>[2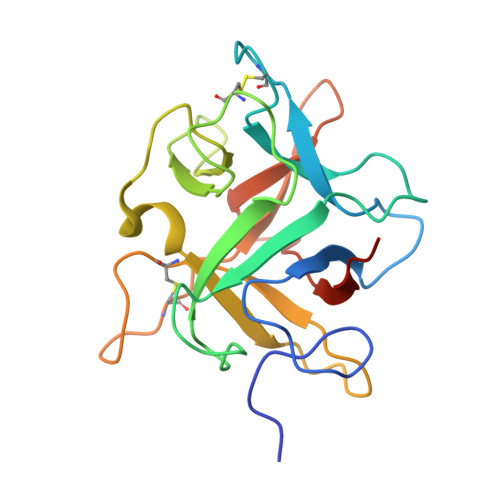x]GSHMDDDLVDAEGNLVENGGTYYLLPHIWAHGGGIETAKTGNEPCPLTVVRSPNEVSKGEPIRISSRLRSAFIPRGSLVALGFANPPSCAASPWWTVVDSPQGPAVKLSQQKLPEKDILVFKFEKVSHSNIHVYKLLYCQHDEEDVKCDQYIGIHRDRNGNRRLVVTEENPLELVLLKAKSETASSH>ALYEDPPDQKTSPSGKPATLKICSWNVDGLRAWIKKKGLDWVKEEAPDILCLQETKCSENKLPAELQELPGLSHQYWSAPSDKEGYSGVGLLSRQAPLKVSYGIGDEEHDQEGRVIVAEFDSFVLVTAYVPNAGRGLVRLEYRQRWDEAFRKFLKGLASRKPLVLCGDLNVAHEEIDLRNPKGNKKNAGFTPQERQGFGELLQAVPLADSFRHLYPNTPYAYTFWTYMMNARSKNVGWRLDYFLLSHSLLPALCDSKIRSKALGSDHCPITLYLAL[2x]

Human APE1 is an essential enzyme and multifunctional nuclease with AP-endonuclease, 3′ phosphodiesterase, 3′ to 5′ exonuclease, and RNA cleavage activities. Instead, rAPs are processed by AP-Endonuclease 1 (APE1), a multifunctional enzyme in the base excision repair (BER) pathway. During BER, abasic (AP) sites are first processed by APE1, which cleaves 5′ of the abasic site generating 3′ hydroxyl and 5′ deoxyribose phosphate termini. Here, we utilize enzyme kinetics, X-ray crystallography, and molecular dynamics simulations to provide insight into rAP processing by APE1.

We obtained crystals of both the substrate form (APE1 bound to an uncleaved rAP site) and product form (APE1 bound to a 5′ nicked rAP site), which diffracted to 2.05 and 2.10 Å, respectively. To generate product complex crystals, we rely on APE1 cleavage of the phosphodiester backbone to create a nick 5′ of the rAP site. Similar to observations of the substrate structures, the rAP DNA backbone (green) is shifted compared to the corresponding structure with deoxy-AP DNA (grey), presumably due to the restrained sugar pucker of the rAP site. However, in the case of the product structure, there is also an accompanying 2.8 Å shift of the 5′ phosphate into the metal binding pocket. This reveals that the rAP is in the position normally occupied by a Mg2+. Interestingly, with the shift of the rAP phosphate backbone relative to the active site residues, these interactions are broken in the rAP product structure. Instead, the phosphate group oxygens are in position to interact with the residues that compose the metal binding pocket (E96, D70, D308) (green). Importantly, with the phosphate in this pocket, it cannot simultaneously contain the catalytic metal, therefore there is no metal bound in this structure. Therefore, in APE1 product structures, this pocket is often occupied by Mg2+, suggesting that here the rAP is actually displacing the Mg2+ out or preventing it from efficiently binding to the metal binding pocket. This highlights the conflict between the rAP and binding of the catalytic metal.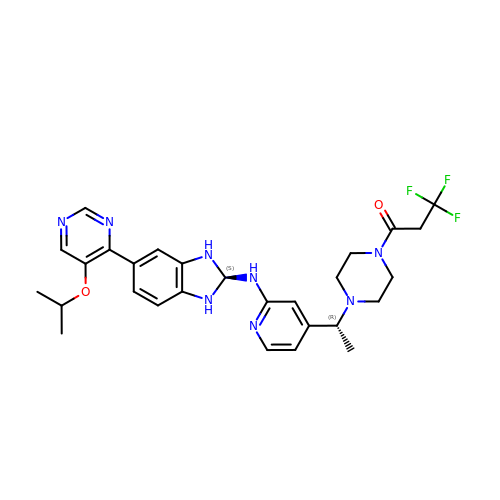3,3,3-tris(fluoranyl)-1-[4-[(1~{R})-1-[2-[[(2~{S})-5-(5-propan-2-yloxypyrimidin-4-yl)-2,3-dihydro-1~{H}-benzimidazol-2-yl]amino]pyridin-4-yl]ethyl]piperazin-1-yl]propan-1-one | C28 H33 F3 N8 O2 | PETZDHZEDSUUQC-CLYVBNDRSA-N>[2x]GQEIRPMPADSAYGVVHISVCNLREEGKFTSGMSTQALLGMPVKVLQYNGWYEIQTPDDYTGWVHR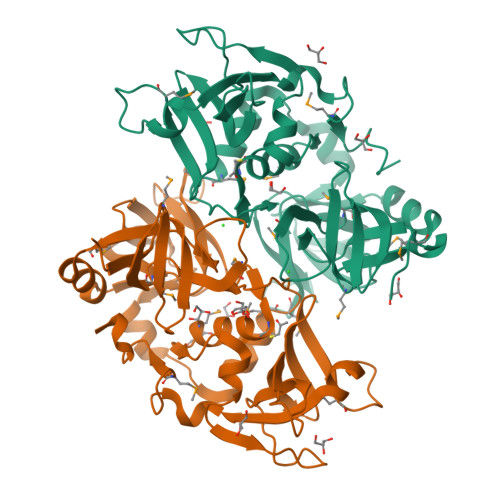MVITPMSKERYDEWNRAEKIVVTSHYGFAYEKPDESSQPVSDVVAGNRLKWEGSKGHFYQVSYPDGRKAYLSKSISQPEAGWRASLKQDVESIIETAYSMMGIPYLWAGTSSKGVDCSGLVRTVLFMHDIIIPRDASQQAYVGEHIDIAPDFSNVKRGDLVFFGRKATAERKEGISHVGIYLGNKQFIHALGDVHVSSMNPADQNYDEFNTKRLLFAVRFLPYINKEKGMNTTNKNPFYQ> MEVCLPNGHQIVDLINNAFEGRVSIYSAQEGWDKTISAQPDMMVCGGAVVCMHCLGVVGSLQRKLKHLPHHRCNQQIRHQDYVDVQFADRVTAHWKRGMLSFVCQMHAMMNDVSPEDLDRVRTEGGSLVELNWLQVDPNSMFRSIHSSWTDPLQVVDDLDTKLDQYWTALNLMIDSSDLVPNF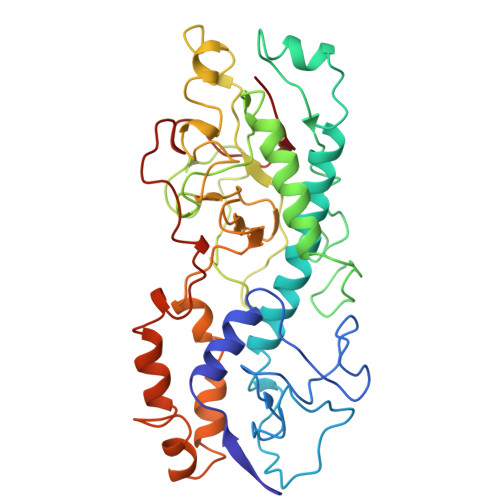MMRDPSHAFNGVRLEGDARQTQFSRTFDSRSSLEWGVMVYDYSELEHDPSKGRAYRKELVTPARDFGHFGLSHYSRATTPILGKMPAVFSGMLTGNCKMYPFIKGTAKLKTVRKLVDSVNHAWGVEKIRYALGPGGMTGWYNRTMQQAPIVLTPAALTMFSDTTKFGDLDYPVMIGDPMILG>[2x]HM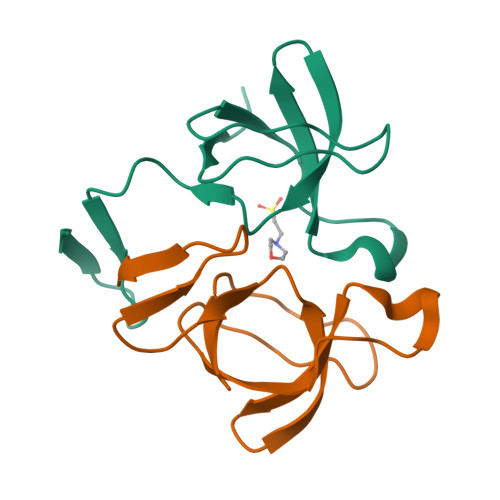YANPVWTALFDYEPSGQDELALRKGDRVEVLSRDAAISGDEGWWAGQVGGQVGIFPSNYVSRGGGAIRINPNGTWSRQAETVES> IVGGKVCPKGECPWQVLLLVNGAQLCGGTLIN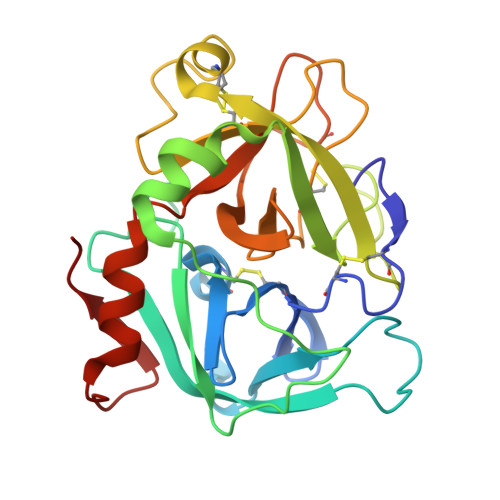TIWVVSAAHCFDKIKNWRNLIAVLGEHDLSEHDGDEQSRRVAQVIIPSTYVPGTTNHDIALLRLHQPVVLTDHVVPLCLPERTFSERTLAFVRFSLVSGWGQLLDRGATALELMVLNVPRLMTQDCEASFPGKITEYMFCAGYSDGSKDSCKGDSGGPHATHYRGTWYLTGIVSWGQGCATVGHFGVYTRVSQYIEWLQKLMRSEPRPGVLLRAPFP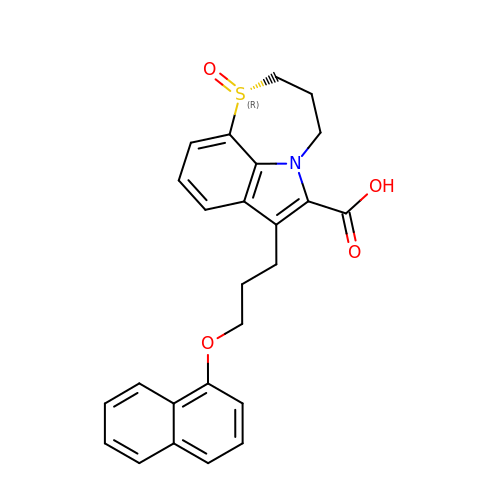(1R)-7-[3-(naphthalen-1-yloxy)propyl]-3,4-dihydro-2H-[1,4]thiazepino[2,3,4-hi]indole-6-carboxylic acid 1-oxide | C25 H23 N O4 S | RWBITVLVWMQUOJ-WJOKGBTCSA-N>MDTSTTASVASANASTSTSMAYDLGSMSKDDVIDLFNKLGVFQAAILMFAYMYQAQSDLSIAKFADMNEASKESTTAQKMANLVDAKIADVQSSSDKNAKAQLPDEVISYINDPRNDITISGIDNINAQLGAGDLQTVKAAISAKANNLTTTVNNSQLEIQQMSNTLNLLTSARSD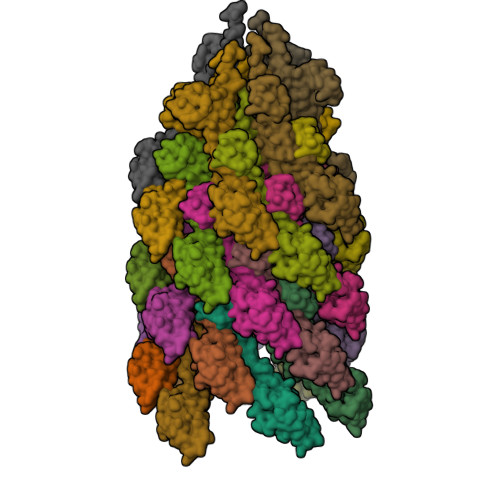MQSLQYRTISGISLGK[28x]>MHTPDCVTGKVEYTKYNDDDTFTVKVGDKELFTNRWNLQSLLLSAQITGMTVTIKTNACHNGGGFSEVIFRGSGSGSGSGSLKTSFKIAFIQARWHADIVDEARKSFVAELAAKTGGSVEVEIFDVPGAYEIPLHAKTLARTGRYAAIVGAAFVIDGGIYRHDFVATAVINGMMQVQLETEVPVLSVVLTPH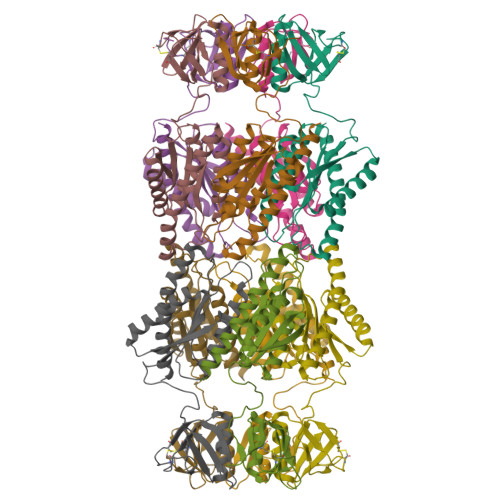HFHESKEHHDFFHAHFKVKGVEAAHAALQIVSERSRIAALV[10x]4-METHYLQUINOLIN-2-AMINE | C10 H10 N2 | 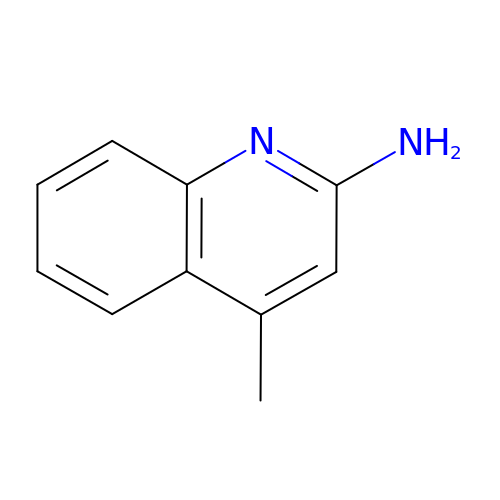LAKQBTPNPXHTNB-UHFFFAOYSA-N> MGAQVSSQKVGAHENSNRAYGGSTINYTTINYYRDSASNAASKQDFAQDPSKFTEPIKDVLIKTAPTLNSPNIEACGYSDRVMQLTLGNSTITTQEAANSVVAYGRWPEYIKDSEANPVDQPTEPDVAACRFYTLDTVTWRKESRGWWWKLPDALKDMGLFGQNMFYHYLGRAGYTVHVQCNASKFHQGALGVFAVPEMCLAGDSTTHMFTKYENANPGEKGGEFKGSFTLDTNATNPARNFCPVDYLFGSGVLAGNAFVYPHQIINLRTNNCATLVLPYVNSLSIDSMTKHNNWGIAILPLAPLD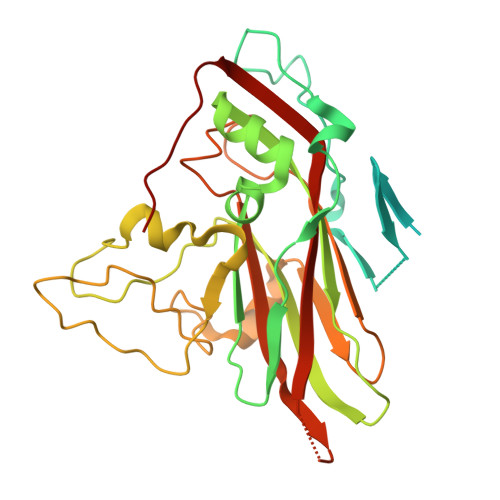FATESSTEIPITLTIAPMCCEFNGLRNITVPRTQ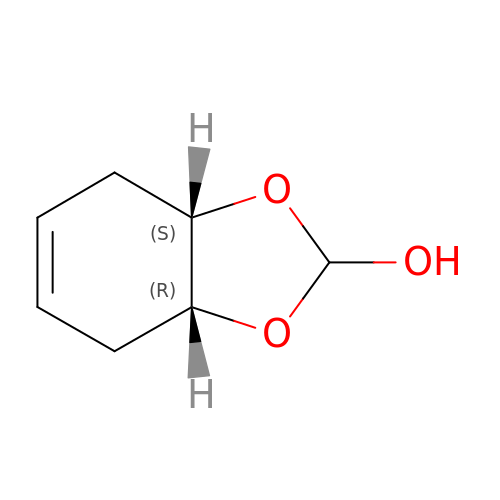3A,4,7,7A-TETRAHYDRO-BENZO [1,3] DIOXOL-2-ONE | C7 H10 O3 | VYBGCFNFGGLKAA-ZMONIFLSSA-N> MERTELLKPRTLADLIRILHELFAGDEVNVE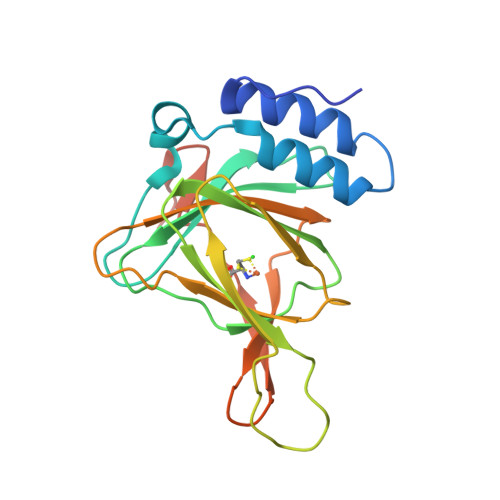EVQAVLEAYESNPAEWALYAKFDQYRYTRNLVDQGNGKFNLMILCWGEGHGSSIHDHTDSHAFLKLLQGNLKETLFDWPDKKSNEMIKKSERTLRENQCAYINDSIGLHRVENVSHTEPAVSLHLYSPPFDTCHAFDQRTGHKNKVTMTFHSKFGIRTPFTTSGSLENN> SGASSAVGGSTRSPSPVDPKRGAVQPRYFITTSLTEKERNSVMEAIQKLGQRAVLVDNKVDEILPLNTTHIVLRGPPRSVAALCGVVSSKWLVQPSYVFDSLGAGFWLDEEVEGGLRYFPPPLRCQRFLLTMPEGVVKTMLQR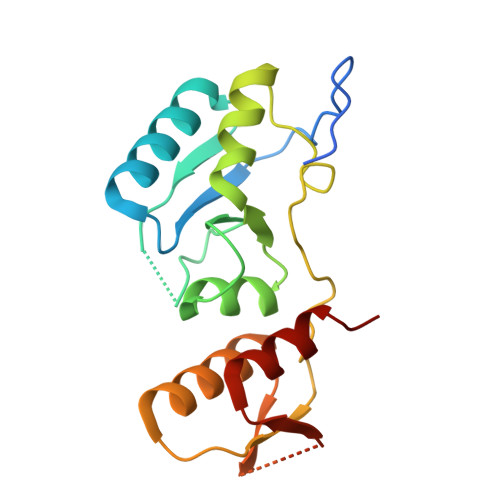VVEFGGGEVVGTKRNGSSNDQDVVVVSSGDELLRFAISRD> GPYAG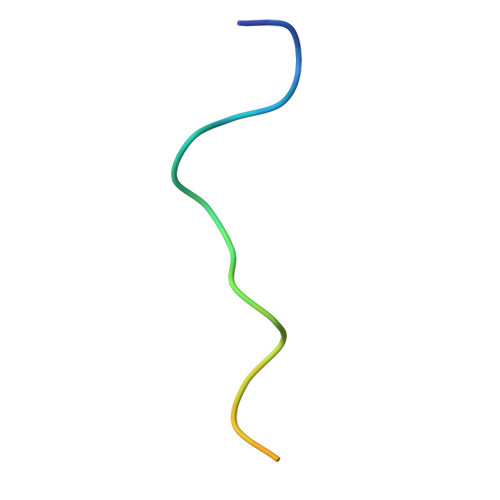PLERQRPLKVKAKLPQAE>[8x]TGGVQTVTLIPGDGIGPEISAAVMKIFDAAKAPIQWEERNVTAIQGPGGKWMIPSEAKESMDKNKMGLKGPLKTPIAAGHPSMNLLLRKTFDLYANVRPCVSIEGYKTPYTDVNIVTIRENTEGEYSGIEHVIVDGVVASIKLITEGASKRIAEFAFEYARNNHRSNVTAVHKANIMRMSDGLFLQKCREVAESCKDIKFNEMYLDTVCLNMVQDPSQFDVLVMPNLYGDILSDLCAGLIGGLGVTPSGNIGANGVAIFESVHGTAPDIAGKDMANPTALLLSAVMMLRHMGLFDHAARIEAACFATIKDGKSLTKDLGGNAKCSDFTEEICRRVKDLD;>ASRSQAEDVRVEGSFPVTMLPGDGVGPELMHAVKEVFKAAAVPVEFQEHHLSEVQNMASEEKLEQVLSSMKENKVAIIGKIHTPMEYKGELASYDMRLRRKLDLFANVVHVKSLPGYMTRHNNLDLVIIREQTEGEYSSLEHESARGVIECLKIVTRAKSQRIAKFAFDYATKKGRGKVTAVHKANIMKLGDGLFLQCCEEVAELYPKIKFETMIIDNCCMQLVQNPYQFDVLVMPNLYGNIIDNLAAGLVGGAGVVPGESYSAEYAVFETGARHPFAQAVGRNIANPTAMLLSASNMLRHLNLEYHSSMIADAVKKVIKVGKVRTSDMGGYATCHDFTEEICRRVKDLDEN[8x]

Human NAD-dependent isocitrate dehydrogenase or IDH3 (HsIDH3) catalyzes the decarboxylation of isocitrate into α-ketoglutarate in the tricarboxylic acid cycle. It consists of three types of subunits (α, β, and γ) and exists and functions as the (αβαγ)2 heterooctamer. HsIDH3 is regulated allosterically and/or competitively by numerous metabolites including CIT, ADP, ATP, and NADH. In this work, we report the crystal structures of the αβ and αγ heterodimers and the (αβαγ)2 heterooctamer containing an α-Q139A mutation in the clasp domain, which renders all the heterodimers and the heterooctamer constitutively active in the absence of activators.

Crystals of the apo αMβ belong to space group C21, and the asymmetry unit contains eight αMβ heterodimers, which form four (αMβ)2 heterotetramers through noncrystallographic 2-fold axes. In the apo αMβ structure, the conformations of the β3B-α3B and β12B-α8B loops are similar to those in the WT αβ heterodimer. In the αβ, αMβ, and αMMgβADP structures, the active site assumes an “open” conformation due to the absence of substrate and/or cofactor. However, in all of the αMβ structures, the hydrogen-bonding network at the αβ-αβ interface is similar to that in the αMgγMg+CIT structure or the αMγ structures, indicative of active conformations. In the αMβ structures, the α-Q139A mutation eliminates the Gln139A1-Gln139A2 hydrogen bond. The intramolecular hydrogen bonds His131A1-Gln139A1 and His131A2-Gln139A2 are replaced by the intermolecular hydrogen bonds His131A1-His142B2 and His131A2-His142B1, and in addition, His142B1 and His142B2 form extra hydrogen bonds with Glu150B1 and Glu150B2. The changes of hydrogen-bonding interactions at the αβ-αβ interface induce conformational changes of the β5-β6 loops, which lead the sidechains of Tyr126A and Tyr137B to adopt the active conformations as well. The results show that in the absence of activators, both αMβ and αMγ heterodimers exhibit significantly higher Vmax and lower S0.5,ICT compared to those of the WT αβ and αγ heterodimers. In contrast to the WT αβ and αγ heterodimers, both of which exist as heterodimers (75 kDa) at low concentration and a dimer of heterodimers or heterotetramer [(αβ)2 and (αγ)2] (130 kDa) at high concentration, the mutant heterodimers exhibit an average molecular mass of approximately 131 to 149 kDa at both low and high concentrations, corresponding to a heterotetramer [(αMβ)2 and (αMγ)2].Of particular interest in this regard is the putative centriolar CPAP–STIL complex, as mutations in both components result in MCPH. CPAP and STIL are strictly required for centriole assembly: STIL at a very early stage and CPAP slightly later, possibly by controlling the organisation and length of the centriolar microtubules. Instead, we demonstrate that the TCP domain of CPAP constitutes a novel proline-rich-motif (PRM) recognition-domain that specifically binds to a short target motif in STIL. Our mutational analysis of the interface demonstrates a remarkable correlation between the ability of mutant proteins to bind to one another in vitro and their ability to support centriole assembly in vivo, providing compelling support for our structural model of the metazoan CPAP–STIL complex. These data strongly suggest that the interaction between CPAP and STIL is a conserved, essential step in centriole biogenesis.

To understand how CPAP and STIL interact at the molecular level, we obtained the crystal structures of the TCP-domain of D. rerio CPAP937–1124, both on its own and in a complex with D. rerio STIL408–428. In both structures, the TCP domain adopts a nearly identical conformation, suggesting that no significant conformational change occurs in CPAP upon binding to STIL (RMSD = 1.5 Å ± 0.2 Å over 148 ± 4 Cα pairs). The TCP domain folds into a single layer β-sheet comprising ∼20 consecutive antiparallel strands connected by type I β-turns and is stabilised by an extensive hydrogen-bonding network. The resulting sheet shows a twist of approximately 13° (i.e., the angle between the consecutive, hydrogen-bonded strands), slightly lower than the average value of 20° observed for typical β-sheets. Individual β-hairpins correspond to previously noted repeats in the TCP domain sequence; the turns of these hairpins are often constituted by a PDG motif explaining the high frequency of proline and glycine residues in this domain. Crystal packing interactions involve only small protein interfaces, suggesting that the protein is biologically active as a monomer. Indeed both small-angle X-ray scattering (SAXS) and size-exclusion chromatography—multi angle light scattering (SEC-MALS) experiments demonstrate that the TCP domain is predominantly monomeric in solution. The structure of the TCP domain represents an unusual, novel architecture. The TCP domain structure lacks a defined hydrophobic core typical for globular domains, and both sides of its β-sheet are exposed to the solvent and well hydrated. However, what, to our knowledge, makes the TCP domain structure unique amongst naturally occurring proteins is that it solely consists of a freestanding meander β-sheet that entirely lacks a defined hydrophobic core and is not flanked by other globular domains that pack against it.

> GPHMEEIMQSDSKIEKMLPDGGRLVVFPNGTRKELSADGQTVKVMFFNGDVKHTMPDQRVIYYYAEAQTTHITYPDGMEVLQFPNNQTEKHFPDGRKEITFPDQTVKTLHPDGREESVLTDGTIIQLNPDGSKVIQFNTGQREIHTADFKRREYPDGTVKTVYSDGRQETQYPTGRVRLKDPQGKVIMDTKA>[2x]GANRTLIVTTILEEPYVMYRKSDKPLYGNDRFEGYCLDLLKELSNILGFLYDVKLVPDGKYGAQNDKGEWNGMVKELIDHRADLAVAPLTITYVREKVIDFSKPFMTLGISILYRKGTPIDSADDLAKQTKIEYGAVRDGSTMTFFKKSKISTYEKMWAFMSSRQQSALVKNSDEGIQRVLTTDYALLMESTSIEYVTQRNCNLTQIGGLIDSKGYGVGTPIGSPYRDKITIAILQLQEEGKL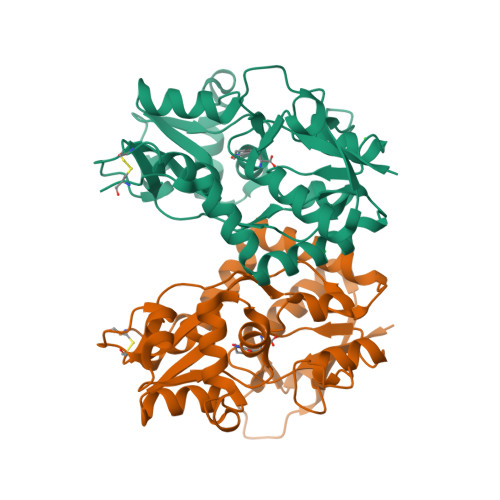HMMKEKWWRGNGCPE>[8x]MGKMAAAVGSVATLATEPGEDAFRKLFRFYRQSRPGTADLEGVIDFSAAHAARGKGPGAQ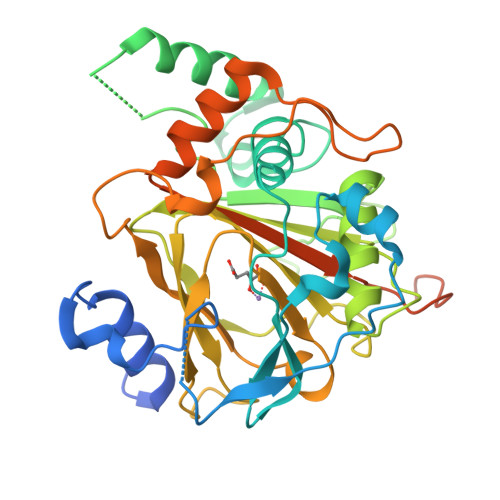KVIKSQLNVSSVSEQNAYRAGLQPVSKWQAYGLKGYPGFIFIPNPFLPGYQWHWVKQCLKLYSQKPNVCNLDKHMSKEETQDLWEQSKEFLRYKEATKRRPRSLLEKLRWVTVGYHYNWDSKKYSADHYTPFPSDLGFLSEQVAAACGFEDFRAEAGILNYYRLDSTLGIHVDRSELDHSKPLLSFSFGQSAIFLLGGLQRDEAPTAMFMHSGDIMIMSGFSRLLNHAVPRVLPNPEGEGLPHCLEAPLPAVLPRDSMVEPCSMEDWQVCASYLKTARVNMTVRQVLATDQNFPLEPIEDEKRDISTEGFCHLDDQNSEVKRARINPDS The lipid-enveloped bacteriophages of the Cystoviridae family infect Gram-negative bacteria, mainly plant-pathogenic Pseudomonas species and share similarities with the members of the Reoviridae family, including bluetongue virus and rotavirus. Their genome of ∼14 kb consists of three dsRNA segments small (S), medium (M) and large (L), which are sequentially encapsidated as ssRNA precursors into the icosahedrally symmetric procapsid by the packaging NTPase P4 (15–23). P4 is a protein of ∼35 kDa, which can assemble into a hexameric ring. NTP-binding sites are located on the external perimeter of the ring at the interfaces between adjacent subunits, whereas the nucleic acid binding sites are found in the central channel. P4 proteins are the only known RNA-specific helicases belonging to helicase Superfamily 4 (SF4).

To understand this catalytic mechanism in detail, we performed side-directed mutagenesis of the residues in ɸ12 P4 involved in binding the nucleotide ring and analysed the mutants structurally and biochemically. In ɸ12 P4 (31), as in RepA, the nucleotide base is sandwiched between Y288 from the catalytic subunit and Q278 from the neighbouring subunit. However, the mutation Q278A had only a moderate effect on ATPase activity and virtually no effect on the structure of the bound ATP analogue AMPcPP when compared with the wild-type, primarily increasing the KM as a result of reduced nucleotide affinity. Hence, the stacking interactions primarily determine nucleotide affinity but not specificity.

>[3x]MIHLYDAKSFAKLRAAQYAAFHTDAPGSWFDHTSGVLESVEDGTPVLAIGVESGDAIVFDKNAQRIVAYKEKSVKAEDGSVSVVQVENGFMKQGHRGWLVDLTGELVGCSPVVAEFGGHRYASGMVIVTGKGNSGKTPLVHALGEALGGKDKYATVRFGEPLSGYNTDFNVFVDDIARAMLQHRVIVIDSLKNVIGAAGGNTTSGGISRGAFDLLSDIGAMAASRGCVVIASLNPTSNDDKIVELVKEASRSNSTSLVISTDVDGEWQVLTRTGEGLARLTHTLQTSYGEHSVLTIHTSKQSGGKQASGKAIQTVIKNDELESVLRRLTSN> MSIDWEQTFRKWSKPSSETESTKAENAERMIKAAINSSQILSTKDISVFPQGSYRNNTNVREDSDVDICVCLNTLVLSDYSLVPGMNDKLAELRTASYTYKQFKSDLETALKNKFGTL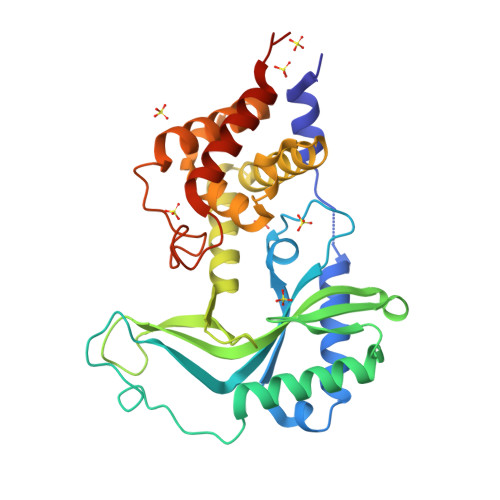GVSRGDKAFDVHANSYRVDADVVPAIQGRLYYDKNHNAFIRGTCIKPDSGGTIYNWPEQNYSNGVNKNKSTGNRFKLIVRAIKRLRNHLAEKGYNTAKPIPSYLMECLVYIVPDQYFTGDSYKTNVENCINYLYNQIDSSDWTEINEIKYLFGSHQMWNKTQVKEFLLTAWSYIQKNLEHHHHHH>[4x]MTGGTGADAASAGASSTRPELRGERCLPPAGPVKVTPDDPRYLNLKLRGANSRFNGEPDYIHLVGSTQQVADAVEETVRTGKRVAVRSGGHCFEDFVDNPDVKVIIDMSLLTEIAYDPSMNAFLIEPGNTLSEVYEKLYLGWNVTIPGGVCGGVGVGGHICGGGYGPLSRQFGSVVDYLYAVEVVVVNKQGKARVIVATRERD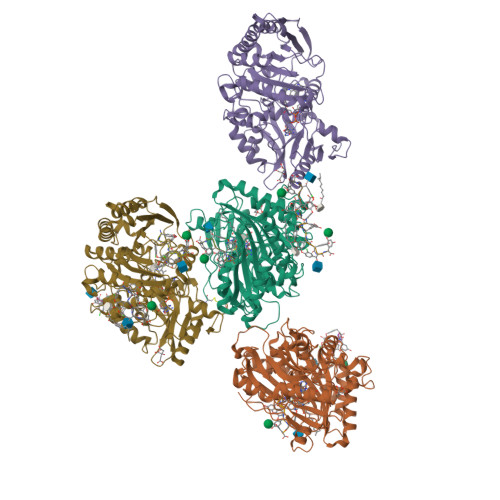DPHHDLWWAHTGGGGGNFGVVTKYWMRVPEDVGRNPERLLPKPPATLLTSTVTFDWAGMTEAAFSRLLRNHGEWYERNSGPDSPYTGLWSQLMIGNEVPGMGESGFMMPIQVDATRPDARRLLDAHIEAVIDGVPPAEVPEPIEQRWLASTPGRGGRGPASKTKAGYLRKRLTDRQIQAVYENMTHMDGIDYGAVWLIGYGGKVNTVDPAATALPQRDAILKVNYITGWANPGNEAKHLTWVRKLYADVYAETGGVPVPNDVSDGAYINYPDSDLADPGLNTSGVPWHDLYYKGNHPRLRKVKAAYDPRNHFHHALSIRP>MKGFAMLSIGKVGWIEKEKPAPGPFDAIVRPLAVAPCTSDIHTVFEGAIGERHNMILGHEAVGEVVEVGSEVKDFKPGDRVVVPAITPDWRTSEVQRGYHQHSGGMLAGWKFSNVKDGVFGEFFHVNDADMNLAHLPKEIPLEAAVMIPDMMTTGFHGAELADIELGATVAVLGIGPVGLMAVAGAKLRGAGRIIAVGSRPVCVDAAKYYGATDIVNYKDGPIESQIMNLTEGKGVDAAIIAGGNADIMATAVKIVKPGGTIANVNYFGEGEVLPVPRLEWGC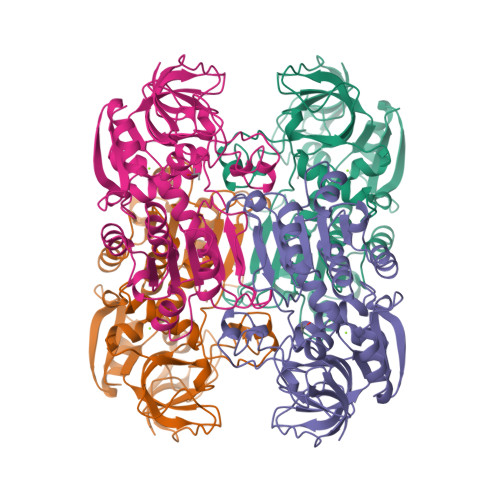GMAHKTIKGGLCPGGRLRMERLIDLVFYKRVDPSKLVTHVFRGFDNIEKAFMLMKDKPKDLIKPVVILA[4x]>MHHHHHHVKLQLVAVGTKMPDWVQTGFTEYLRRFPKDMPFELIEIPAGKRGKNADIKRILDKEGEQMLAAAGKNRIVTLDIPGKPWDTP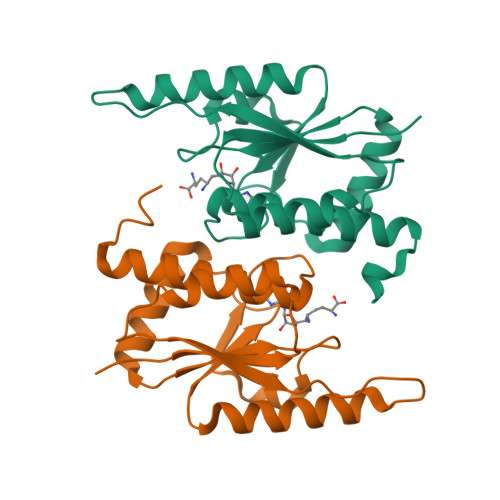QLAAELERWKLDGRDVSLLIGGPEGLSPACKAAAEQSWSLSALTLPHPLVRVLVAESLYRAWSITTNHPYHRE[4x]>[2x]MSLTLFHNPASPYVRKVMVLLHETGQLNRVALQASQLSPVA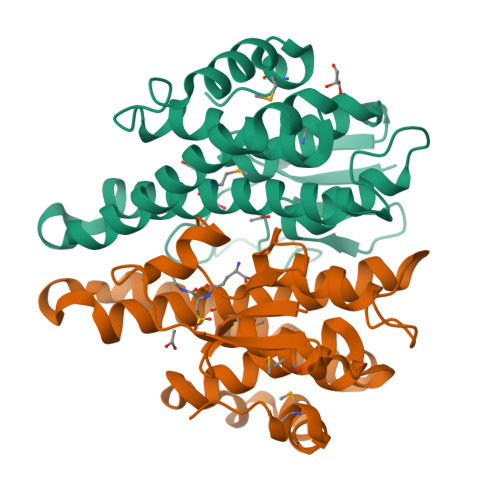PDAALNQDNPLGKIPALRLDNGQVLYDSRVILDYLDQQHVGNPLIPRDGSARWRRLTLAALADGIMDASVLVRYELALRAPEKHWEQWLDGQRDKIRRALAVLEAEAIAELASHFDIAAISVACALGYLDFRHPDLEWRQDHPQLAAWYFEISQRPSMLATRPPVEGHHHHHH>GTAPKVLFTGVVDARGERAVLALGGSLAGSAAEASHLVTDRIRRTVKFLCALGRGIPILSLDWLHQSRKAGFFLPPDEYVVTDPEQEKNFGFSLQDALSRARERRLLEGYEIYVTPGVQPPPPQMGEIISCCGGTYLPSMPRSYKPQRVVITCPQDFPHCSIPLRVGLPLLSPEF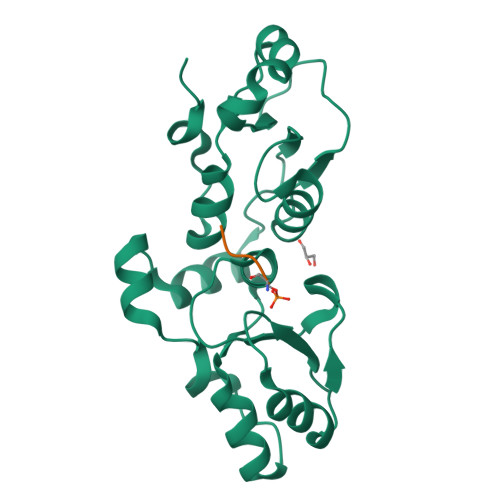LLDGVLKQEAKPEAFVLSPLEMSST[2x];>SQEYX[2x]>[4x]ARPCIPKSFGYSSVVCVCNATYCDSFDPPTFPALGTFSRYESTRSGRRMELSMGPIQANHTGTGLLLTLQPEQKFQKVKGFGGAMTDAAALNILALSPPAQNLLLKSYFSEEGIGYNIIRVPMASCDFSIRTYTYADTPDDFQLHNFSLPEEDTKLKIPLIHRALQLAQRPVSLLASPWTSPTWLKTNGAVNGKGSLKGQPGDIYHQTWARYFVKFLDAYAEHKLQFWAVTAENEPSAGLLSGY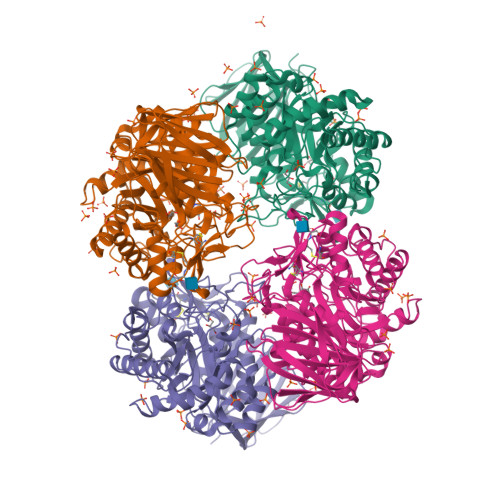PFQCLGFTPEHQRDFIARDLGPTLANSTHHNVRLLMLDDQRLLLPHWAKVVLTDPEAAKYVHGIAVHWYLDFLAPAKATLGETHRLFPNTMLFASEACVGSKFWEQSVRLGSWDRGMQYSHSIITNLLYHVVGWTDWNLALNPEGGPNWVRNFVDSPIIVDITKDTFYKQPMFYHLGHFSKFIPEGSQRVGLVASQKNDLDAVALMHPDGSAVVVVLNRSSKDVPLTIKDPAVGFLETISPGYSIHTYLWHRQ>[2x]GAMDDIDEEDDDLVGVSVRPKVPLRTMSYKLAIDMSHFIKEKGGLEGIYYSARRHRILDIYLEKEEGIIPDWQDYTSGPGIRYPKTFGWLWKLVPVNVSDE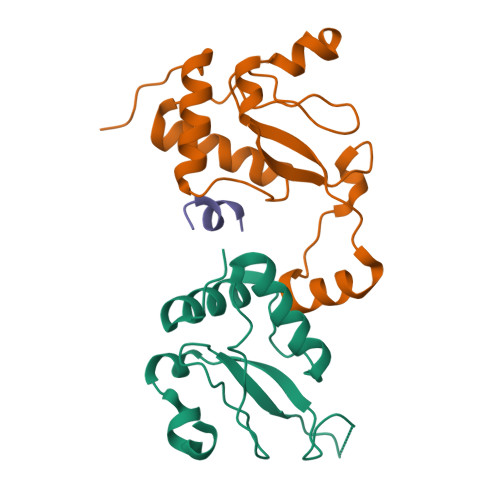AQEDEEHYLMHPAQTSQWDDPWGEVLAWKFDPTLAYTYEAYVRYPEEFGS> MSQKDNLLDNPVEFLKEVRESFDIQQDVDAMKRIRHDLDVIKEESEARLKLYRSLGVILDLENDQVLINR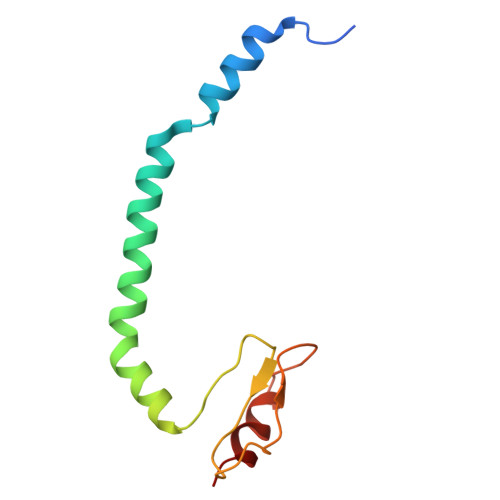KNDGNIDILPLDNNLSDFYKTKYIWERLG>MLTEFDAGYGEQPFRDLCANYPGAEAYDPHDFRIEWGPIFHRGRLDGSARVLIVGQDPAQHETIVRRILVGTAGRRTQGFLAKLGIVQSYVMVNTFLYSVYGQSGGSKHKNEPGIVDYRNKWFKAVLGPGNIEAVVSLGGLADEAWKA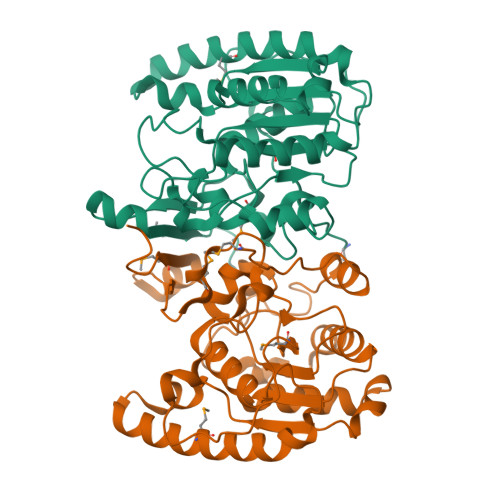WLKSSDGAAYKTLAYQHITHPTWPESSAHDSATQAANTKIMLAKWNAALAALAPEVKHPDVPTTLVPYGDAFKPSELVDIIAKDLPAGLPAWMRGDTPWAVRQGVDAAAKRRTIMITIPDGVIP[4x]Several natural systems exhibit ‘facilitated dissociation’, in which an effector (E) can bind to a target–host (TH) complex to form an excited ternary complex (THE)20–26 from which the target dissociates quickly. We set out to design protein systems that undergo facilitated dissociation. We use a switchable target binder (host) and a flexible effector that can rapidly bind to and switch the target–host complex to induce a large steric clash with the target, forming a strained excited ternary complex. We show here that by explicitly considering excited intermediate states when designing coupled protein systems, a broad range of facilitated dissociation systems can be designed.

We used X-ray crystallography to structurally characterize multiple states of our designed systems. The unbound structures show an open hydrophobic cleft in the new designed state X poised to bind the effector, and the effector-bound structures show that binding the effector causes the two switch domains to register-shift into the designed state Y. Structures of the target–AS1 complex show that the target binds as designed (top), with some strain suggested by small variations among the structures (bottom). For (1), the target dissociates 20-fold faster from AS1 than from an unhindered binder fusion, probably because of minor strain in the target–AS1 complex.

>[2x]MSGSMKEEIKRLAEELKEKTKNEEIKRLAEEAAELAERSDDPEVLEVVKKALEEALKSKNEEKIELLLLVAVLVAEAGSVDAVEEKLEIALLALKLAEESKDPRIIRGALRAAIAALRSDDPLALKTVKEALERARASKDERLIRAILAAAYAFALLAVAGASAERLKEAEAIVKELIAAAEKGASPQELVLLVIEMMVKGMGVTMETHRSGNEVKVVIKGLHESQQEVLLEAVLFAAELMGVRVRIRFKGDTVTIVVREGSG;>[2x]MSGEEAVRRRFEELLREALAFRERTGGRRETLEHAVRLARELAEFAASHPEFNRQEAVLLAIELMVRAMGVTMETHRSGNEVKVVIKGLNIDEQVALYRAVRETSKIMGVETEIEVEGDTQTIVVREGSG> DDLNIKTMIPGVPQIDAESYILIDYNSGKVLAEQNADVRRDPASLTKMMTSYVIGQAMKAGKFKETDLVTIGNDAWATGNPVFKGSSLMFLKPGMQVPVSQLIRGINLQSGNDACVAMADFAAGSQDAFVGLMNSYVNALGLKNTHFQTVHGLDADGQYSSARDMALIGQALIRDVPNEYSIYKEKEFTFNGIRQLNRNGLLWDNSLNVDGIKTGHTDKAGYNLVASATEGQMRLISAVMGGRTFKGREAESKKLLTWGFRFFETVNPL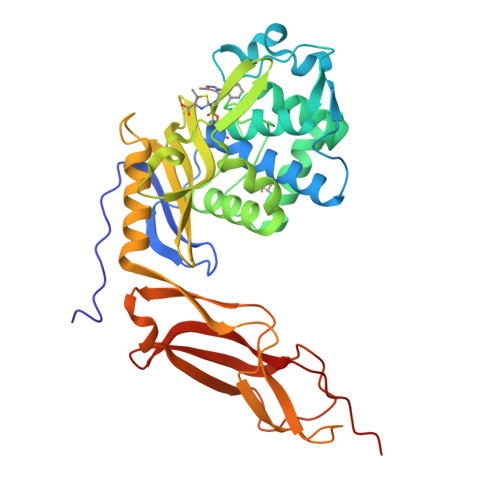KVGKEFASEPVWFGDSDRASLGVDKDVYLTIPRGRMKDLKASYVLNSSELHAPLQKNQVVGTINFQLDGKTIEQRPLVVLQEIPEGNFGDPVID>MPAKSPVIVDLKFIPEEVEAALAGAFPGREVIDLADPAHQERDLSGIDYAVVWKSAPDLFSRAPDLKVVFSGGAGVDHVLTLPGLPDVPLVRFVDRTLTTRMSEWVMMQCLLHLRQHRAYEALAKKHEWRDLSQPEAADVTVGIMGMGVLGQDAARKLAAMGFKVIGWSRSKRVIEGVETYDAAGLDAFLGRTDFLVGLLPLTPDTRGIFNAALFAKLSRNGPFGAPVFINAGRGGSQVEADILECLDSGVLGGASLDVFEREPLSPESRFW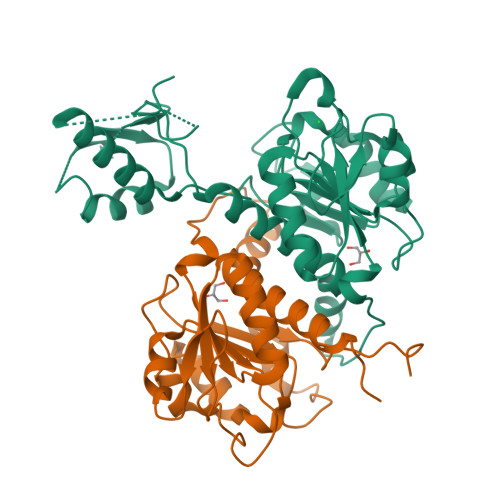DMPNVYVTPHVAASSDVRALFVHVEHQIARFESGLPLEHVVDKVAGY[2x]> EDIDVILKKSTILNLDINNDIISDISGFNSSVITYPDAQLVPGINGKAIHLVNNEESEVIVHKAMDIEYNDMFNNFTVSFWLRVPKVSASHLEQYGTNEYSIISSMKKHSLSIGSGWSVSLKGNNLIWTLKDSAGEVRQITFRDLPDKFNAYLANKWVFITITNDRLS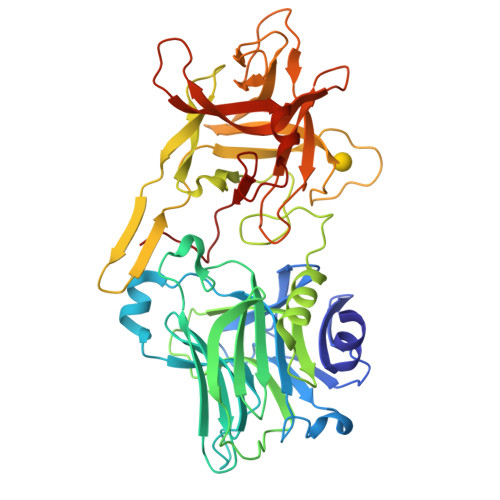SANLYINGVLMGSAEITGLGAIREDNNITLKLDRCNNNNQYVSIDKFRIFCKALNPKEIEKLYTSYLSITFLRDFWGNPLRYDTEYYLIPVASSSKDVQLKNITDYMYLTNAPSYTNGKLNIYYRRLYNGLKFIIKRYTPNNEIDSFVKSGDFIKLYVSYNNNEHIVGYPKDGNAFNNLDRILRVGYNAPGIPLYKKMEAVKLRDLKTYSVQLKLYDDKNASLGLVGTHNGQIGNDPNRDILIASNWYFNHLKDKILGCDWYFVPTDEGWTND>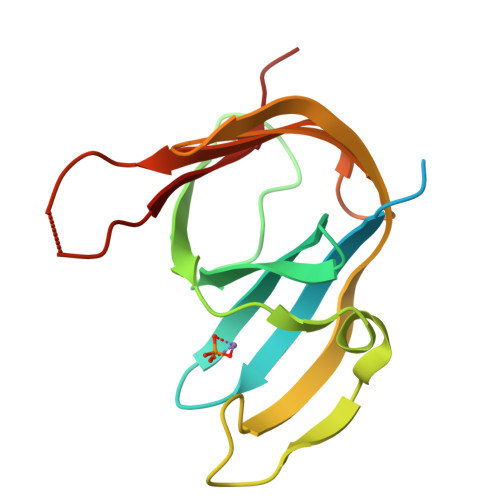 SMLEEYEKKRHFQKTPEPSTTGVKKSSDKPIFVVQRHDARKLHYDFRLEMDGVLKSWAVPKEPPKDAGTRRLAIETEDHPLAYADFEGEIPAGEYGAGKVEIWDRGTFELLKREEREIVVSLEGKELKGIYVLIRTKYGKGEKGWLFFKKAS> MITMKCRKCGKPSIYHQKHSGNNYCKECFIKETKRKVRKTLGRDVLKNNIKVAMGLSGGKDSLVMAYLLNEYYKQIPNSNLIAIMVNEGIEGYRTDGIDAAVKFCEEYGIEYKIVHFKDYLGTNLDEIVKIAKEKNLTMNPCSFCGVIRRKILNRVSIEEKCDFLAIGHNLDDVAQAVMMNYIEGDVKKLAFLGKSLKHPKFVKRIKPLEKIPEDEVLLLAEMLELKYHKSPCPYSCLSFRSEVSDITDNLEKNHPGSKYSIVRGYERLLEHIELPGYTGECKICGDLSATEVCKVCSYLKNLGILEK;> MITMKCRKCGKPSIYHQKHSGNNYCKECFIKETKRKVRKTLGRDVLKNNIKVAMGLSGGKDSLVMAYLLNEYYKQIPNSNLIAIMVNEGIEGYRTDGIDAAVKFCEEYGIEYKIVHFKDYLGTNLDEIVKIAKEKNLTMNPCSFCGVIRRKILNRVSIEEKCDFLAIGHNLDDVAQAVMMNYIEGDVKKLAFLGKSLKHPKFVKRIKPLEKIPEDEVLLLAEMLELKYHKSPCPYSCLSFRSEVSDITDNLEKNHPGSKYSIVRGYERLLEHIELPGYTGECKICGGLSATEVCKVCSYGKNLGILEKSKF

Thiolation of uridine 34 in the anticodon loop of several tRNAs is conserved in the three domains of life and guarantees fidelity of protein translation. U34-tRNA thiolation is catalyzed by a complex of two proteins in the eukaryotic cytosol (named Ctu1/Ctu2 in humans), but by a single NcsA enzyme in archaea. We report here spectroscopic and biochemical experiments showing that NcsA from Methanococcus maripaludis (MmNcsA) is a dimer that binds a [4Fe-4S] cluster, which is required for catalysis. We thus propose that the same mechanism for U34-tRNA thiolation, mediated by a [4Fe-4S]-dependent enzyme, operates in archaea and eukaryotes.

The crystals belong to space group P212121 and contain two molecules in the asymmetric unit that form a dimer. The [4Fe-4S] cluster is chelated by three conserved cysteines only: Cys142, Cys145, and Cys233. Remarkably, while three Fe atoms are attached to the protein via these 3 cysteines, the fourth iron completes its coordination with a non-protein, exogenous ligand, as revealed by an electron density adjacent to that Fe atom. Based on the diffraction data at only one wavelength, it is not possible to distinguish between a water molecule, a hydrogenosulfide ion, a chloride ion or the oxygen atom of a sulfate molecule, which all could be refined with B-factors in the same range as those for the protein. Note that several sulfate ions originating from the crystallization solution were observed within the active site. A negatively charged ligand on the fourth iron atom is very likely, given its charge complementary with the [4Fe-4S]2+ cluster and its proximity with the guanidinium group of Arg149, located less than 3 Å away. Superposition of the MmNcsA and PhTtuA catalytic cores shows that the two proteins adopt the same fold but highlights different orientations of the terminal zinc-containing domains relative to the catalytic core. Moreover, Lys135 in PhTtuA is replaced, in MmNcsA, by Arg149 that adopts two different conformations. In both molecules of the asymmetric unit, two loops (residues 130–137 and 275–280), for which there was no electron density, were not modelled. The propensity of the fourth non protein-bonded iron to bind a small molecule indicates that the [4Fe-4S] cluster likely plays a direct role as a Lewis acid in catalysis, specifically to bind, activate a HS− species and transfer it to the activated substrate, as proposed earlier for TtuA39.>MSSELSA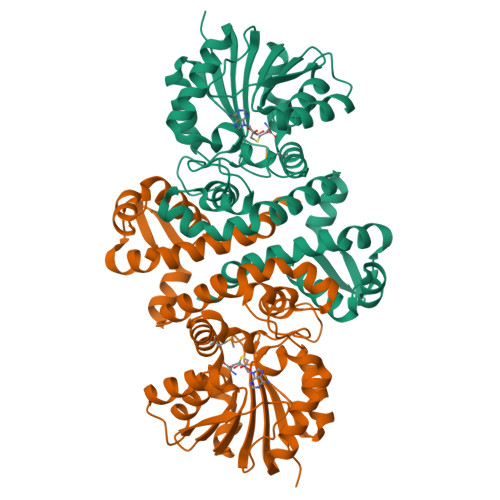LVPVLFGHAAFQQLNAGCQLGLFELLHERGPLSAEEVADALRLPRRSADILLLGTTALGLSTVTDGGYRNGAPIGAAFRDGLWPVLRDIVQYQDKIAYQPAADYVESLRTGQNAGIRHFPGTTRDLYSRLAAVPGLEELFYRGMHAWSQLSNPVLLAQPDFTRVHRVLDVGGGDAVNAVALARAHPSLRVTVLDRPGALEVARKTIAEAGLEERVRTHAADIFTDSYPAGHDCVLFAHQLVIWSPEQNLTLLRKAYDAVEPGGRVLVFNAFTDDDRTGPLYAALDNVYFTTLPFRHSTIHRWADCESWLREAGFTDVGRTAPPGWTPHGVVSGSRPRAAALEHHHHHH[4x]>[2x]MQGQQKESLESLFTKDSDPTVLDAAEQFAQWTLPTVLTRDISGMDGKRTSLHRDYQSTGAVLVNSASTKVTNALFPQGAPFFRFVDSPDMAAAVAELGINGTVQSQQSQIELSASSLVFSRDNYAASLRAVKLLMV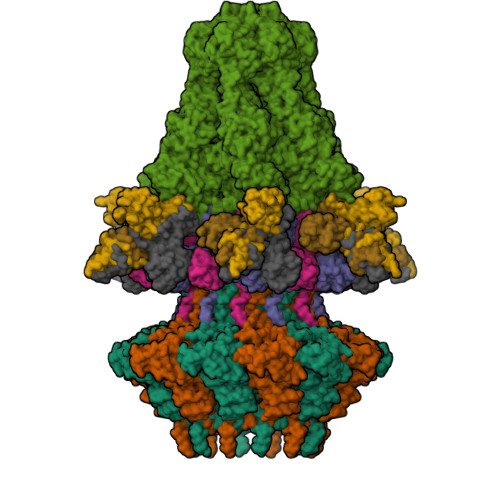TGNALEYFDEGTGRSHIYSVREYTVRRDGSGNILRVVLKERIAAMDLPQEFRSAHLGQKDDYDDVTLYTGICLEDNKFKIYQEVQQQQIGDASTYPIDECPYTVLVWNLVNGEHYGRGLVEDYAGDFARLSVLSQALTLYEVEAARLYNAVSAGAGIDVDAAQAAETGDYVQTSAAPGTNPGIWAVENGSDRKIMSLQSEISMIEQKLARAFMYAGNTRQGERVTAYEIRTNAQEAQNSLGDAYSILSDHWLRKRAYLYTVYQYPPMRAMFTLGATTIQILVGTASLNKAAQADRLLEASQSIQLVLPVLQGATKRTNPDAVVDFILDAFGVVSSKLMYTEEQLKQIQDQQDQQQADQQRNLELAQANPEVAGQQLGLIPS;>[2x]MRLTDAVNVTLEALGESRIVDINTSNPSAGLARAALDRTRRGVLSTGWWFNTIIREVTPTPNPGQIKVPWNQLSMYGLDGTKYGERDGVLYNLVDQTKVFSDTVHLKVVIDIDFEDLPEHMAMWVANATAAQVYLNDLGADGNYKSLLGIAAEYEAMNMREHLRNQRYSTSRTHAARKIRSGFFR;> MAQTFEGTLQSLLQGVSQQIPRERQPGQLGAQQNMLSDPVTGLRRRPPLHLAAQTLMENPVSPDALFSTYIERGTDGRHLLINTEAGIWQILSKDATTLIRSGQADYLKASIGATSIQTASIAGLTYILNTEQTPVAHVDNTGKLNPANTGFFYIVASSFSKRWTITVQSNEGTWTAVHDVGASSDDGAVPAATASAVINSLKTNLLAAGMPSDKVDTFGSYMFIKGLTNVVVSSDAGTTYARWSNQSRVDEESDLPAQLPASANGCMCRVGAASTSATWYRFDYATRQWNEDSAYSSITKITNMPLEFAADDQIIPRDFEGRLAGDDENNEDPGFVENGYITGIAAFQGRLVLLSGSRVSMSASGLYQRFYRSTVVNLLDTDRIDIGAASAQDSVFRAALQFNRDLVVFGDSMQAVIAGNAVLTPTNASIALTSEFSCDSRVIPVVTGQTVLYASRRNSDYAGLLEFIPSAYTSSQYVSQDATVHLPRYIPGRVMDMQVSSVTNVAFFRYSGERTSVLVYEFLWGEDAKRAQGAYHKWVLPYDVLSLHTLSEAAYFFVRGPGAYVLALRVDPREGFVAGTTYEYPFMDMGAPVTVQGGQFTLPEHLRKAGLQDSIALAYYTGDDSGSELGIASISSNWVCTTVRGVPDGNYLAGYRFKSGTTLTPPMLKDQNDNLIGSGHVRLLRLDVAMRNSGVVDVLVEDNARDVDNDSEYSGVLMNSKELAPEQPLKASLSNIIIPCRTNTDTTEVTLSTSGTLEMNIMDVSYILRYNQRRRRV;>MAYSWSEQVVPSGTTLISVDIEYLDKSYIYLYINNVLISNSDYSWNSDTLIQLNTPMASAGTVLLVRRTDKEYLYIMFAEGAAFIRENLDVQNTQFLHLAQELVEGRSIDGFYGDLSMNGYRITHLADGVDPKDAVNKGQLDSVSNRVSSIENSFLGLTTVSYPWYTVVSADTDTFEPPFKFTKAALYIDGLCQVPDYSYVVVDNKLLLAESVPTGTVVFARLGEDTDAATEAATTTALAAVQADLQNQINALRALLQGG[3x]>[2x]MSIDKSYCGFIAIVGRPNVGKSTLLNKLLGQKISITSRKAQTTRHRIVGIHTEGAYQAIYVDTPGLHMEEKRAINRLMNKAASSSIGDVELVIFVVEGTRWTPDDEMVLNKLREGKAPVILAVNKVDNVQEKAD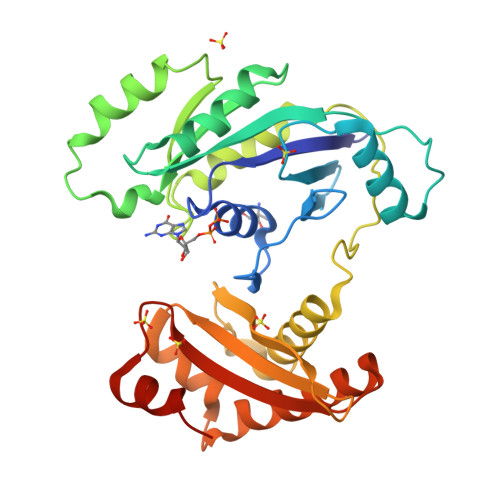LLPHLQFLASQMNFLDIVPISAETGLNVDTIAAIVRKHLPEATHHFPEDYITDRSQRFMASEIIREKLMRFLGAELPYSVTVEIERFVSNERGGYDINGLILVEREGQKKMVIGNKGAKIKTIGIEARKDMQEMFEAPVHLELWVKVKSGWADDERALRSLGYVDDL> AGLATIDELQTLMSTVFEDDALEQAQLVLDIVSSWARVVSGQMWPDAPANVPDDVR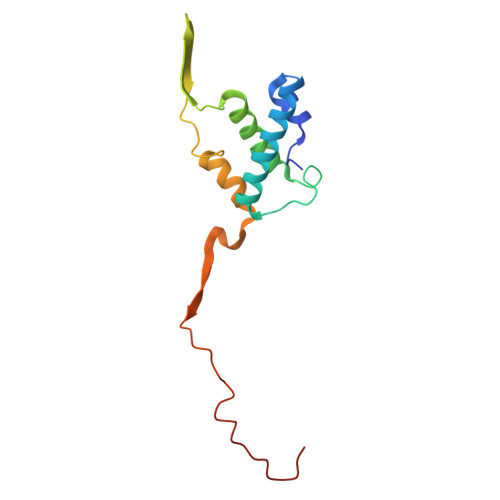AVVLQASRRELKNPDRVISRQMGPFNVQYSQPPDGFFYPAELAILKRFKRSGGLMTVSTSRGEEGRPWAGKTAYIRYGDGL>GPLGSMSVLRPLDKLPGLNTATILLVGTEDALLQQLADSMLKEDCASELKVHLAKSLPLPSSVNRPRIDLIVFVVNLHSKYSLQNTEESLRHVDASFFLGKVCFLATGAGRESHCSIHRHTVVKLAHTYQSPLLYCDLEVEGFRATMA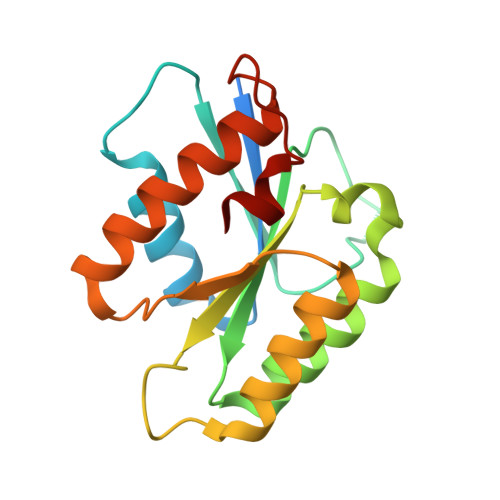QRLVRVLQICAGHVPGVSALNLLSLLRS[2x]> GSHMTRPQAAAEDARNAMVAGLLASGISVNGLQPSHNPQVAAQMFTTATRLDPKMCDAWLARLLAGDQSIEVLAGAWAAVRTFGWETRRLGVTDLQFRPEVSDGLFLRLAITSVDSLACAYAAVLAEAKRYQEAAELLDATDPRHPFDAELVSYVRGVLYFRTKRWPDVLAQFPEATQWRHPELKAAGAAMATTALASLGVFEEAFRRAQEAIEGDRVPGAANIALYT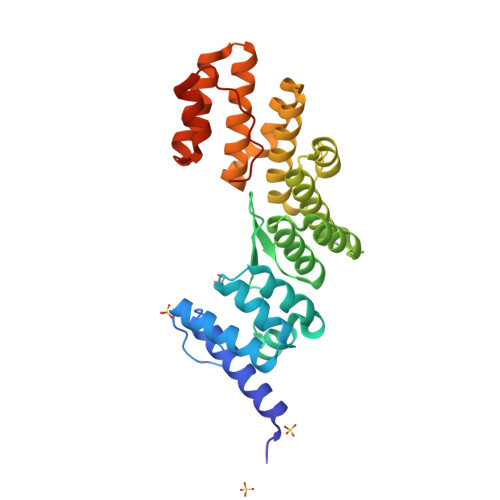QGMCLRHVGREEEAVELLRRVYSRDAKFTPAREALDNPNFRLILTDPETIEAR> MSTSSHTVLLIQTSPRLDSRTWGDYESVTDALDALCKMFEDFLSKKSAAPVTYDVSQVYEFLDKLSDVSMMIFNRETGQYIGRTRAWIKQQVYEMMRGRCQHPGSSGSSGSSGSSGSSGSSGSSNKRITLNERFGVLEKGYTIQA;> MSTSSHTVLLIQTSPRLDSRTWGDYESVTDALDALCKMFEDFLSKKSAAPVTYDVSQVYEFLDKLSDVSMMIFNRETGQYIGRTRAWIKQQVYEMMRGRCQHPG

By using functional proteomics, we and another group independently identified a piRNA biogenesis and chromosome segregation (PICS) complex (also named as PETISCO) that plays important roles in 21U-RNA biogenesis, chromosome segregation and cell division. The PICS complex is composed of TOFU-6, PICS-1 (also names as PID-3), ERH-2 and two mutually exclusive factors, PID-1 and TOST-1. The PID-1 containing complex is functional in piRNA maturation and processes piRNA precursors at 5′ termini via its association with IFE-3, while the TOST-1 containing form is essential for chromosome segregation and cell division in embryos. Complemented by biochemical and mutagenesis experiments, our structural biology data support that PICS is an octamer composed of two copies of each subunit, and unveil the assembly interface within PICS complex.

To understand the molecular mechanism how TOST-1 binds to ERH-2, we made a similar fusion protein by linking ERH-2(1–103) with a fragment of TOST-1(34–54) via a (GSS)6 linker, crystallized the fusion protein, and determined its structure at a 2.20 Å resolution. In the TOST-1-bound structure, the ERH-2 homodimer is similar to that in the PICS-1-bound one. However, only one TOST-1 molecule (aa 35–54) is visible in the structure since the crystal packing prevents the access of the second TOST-1 to the symmetrical site. The TOST-1 fragment (TOST-134–54) adopts a helix structure with two extended ends, and the helix is accommodated into the oval-shape pocket of the ERH-2 dimer. The helix of TOST-1 (aa 39-48) interacts with both ERH-2 protomers, ERH-2A and ERH-2B, via hydrophobic and electrostatic interactions. Leu39, Phe43, and Leu46 of TOST-1 make extensive hydrophobic interactions with Val8A, Trp22A, Phe73A, Tyr80A, Leu10B, and Met71B. The main chain amides of Leu39 and Asn40 form are hydrogen bonded to the carboxyl groups of Asp67B; The side chain carboxyl group of TOST-1 Asn40 is hydrogen bonded to the main chain amide group of Arg85B; The guanidino group of Arg42 forms cation-π and salt bridge with the side chains of His6A and Glu26A, respectively. In addition to the helix-mediated interactions, the Arg36 of TOST-1 forms salt bridge with Asp24A, and the Thr51 of TOST-1 also makes additional hydrophobic contacts with Phe73A. By using ITC binding assay, we found that D67A of ERH-2, R42C and L39A/F43A of TOST-1, abolished the interaction between TOST-1 and ERH-2, whereas the ERH-2 D67A binds to EBM in a comparable affinity with the wild type (Kds: 4.3 μM vs. 8.5 μM). In addition, those mutants abolishing the ERH-2/TOST-1 interaction, including D67A of ERH-2, L39A/F43A and R42C of TOST-1, all demonstrated delay and nondisjunction in chromosome segregation and cell division.> GGSQNVSLQPPPQQLIVQNKTIDLPAVYQLNGGEEANPHAVKVLKELLSGKQSSKKGMLISIGEKGDKSVRKYSRQIPDHKEGYYLSVNEKEIVLAGNDERGTYYALQTFAQLLKDGKLPEVEIKDYPSVRYRGVVEGFYGTPWSHQARLSQLKFYGKNKMNTYIYGPKDDPYHSAPNWRLPYPDKEAAQLQELVAVANENEVDFVWAIHPGQDIKWNKEDRDLLLAKFEKMYQLGVRSFAVFFDDISGEGTNPQKQAELLNYIDEKFAQVKPDINQLVMCPTEYNKSWSNPNGNYLTTLGDKLNPSIQIMWTGDRVISDITRDGISWINERIKRPAYIWWNFPVSDYVRDHLLLGPVYGNDTTIAKEMSGFVTNPMEHAESSKIAIYSVASYAWNPAKYDTWQTWKDAIRTILPSAAEELECFAMHNSDLGPNGHGYRREESMDIQPAAERFLKAFKEGKNYDKADFETLQYTFERMKESADILLMNTENKPLIVEITPWVHQFKLTAEMGEEVLKMVEGRNESYFLRKYNHVKALQQQMFYIDQTSNQNPYQPGVKTATRVIKPLIDRTFATVVKFFNQKFNAHLDATTDYMPHKMISNVEQIKNLPLQVKANRVLISPANEVVKWAAGNSVEIELDAIYPGENIQINFGKDAPCTWGRLEISTDGKEWKTVDLKQKES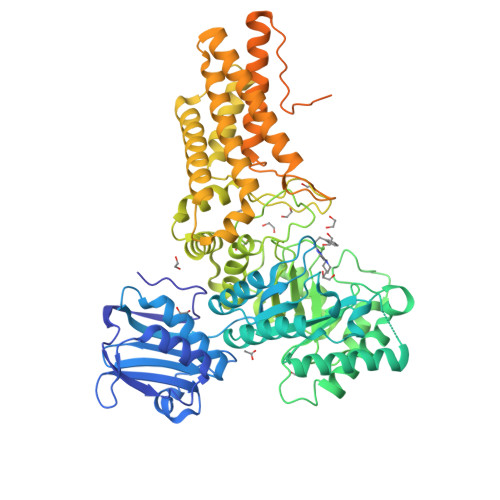RLSAGLQKAPVKFVRFTNVSDEEQQVYLRQFVLTIEKK>MGEEVNFDWHLLLNGYYYSPVDLEVEDIFEIVNQPMDGNCL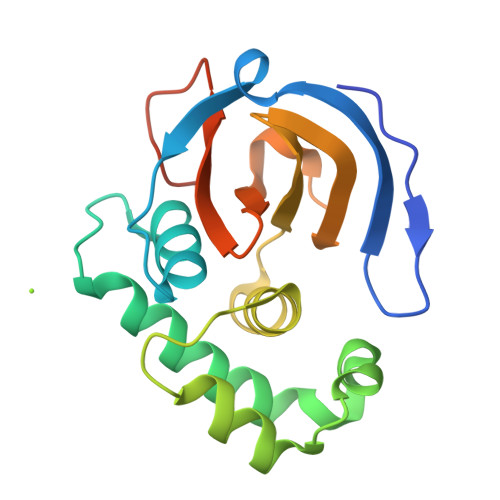YHSLACGMIEEQQPDSYKLIKEQVREAAGLFWDTTEETKTTGEDLNGYLARIMKPNEWGSSLEVNFFSQKAKVTVYIWHEDASKHCDYVVRYGEDPMLESINIMHRRNHYDYLKPRGNQRTAVVKSGSHHHHHH[4x]> MFARAFSRFASLAAPAPQRGWNAFVLPSRHFATAAGGANPFKNQLLLTLSSPSEAIYVRTPVRSVTVPGSEGAMTMTNGHSQTVARLKAGEIIVRKGETGDEVERFFLSDGFVLFKSPE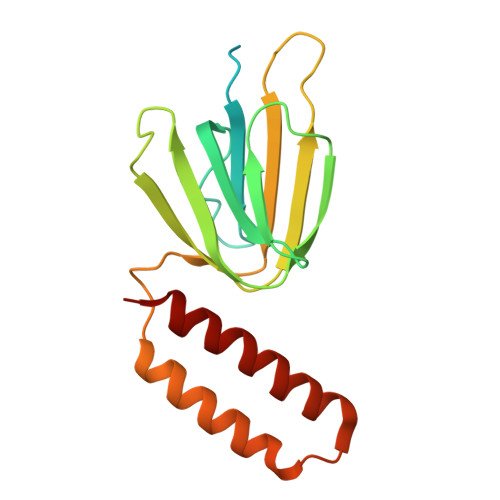DDSGCCTAEVLGVEVVPVSMLDKESAATALQELLQQGAGATDEWTKARTLLGQELLSSVIRAAP> MIPHSWICEKHILWLKDYKNSSNWKLFKECWKQGQPAVVSGVHKKMNISLWKAESISLDFGDHQADLLNCKDSIISNANVKEFWDGFEEVSKRQKNKSGETVVLKLKDWPSGEDFKTMMPARYEDLLKSLPLPEYCNPEGKFNLASHLPGFFVRPDLGPRLCSAYGVVAAKDHDIGTTNLHIEVSDVVNILVYVGIAKG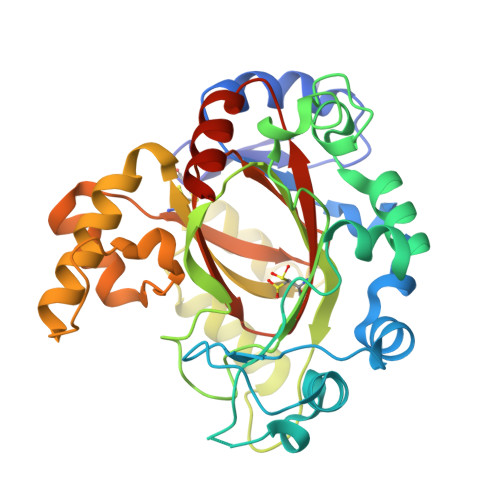NGILSKAGILKKFEEEDLDDILRKRLKDSSEIPGALWHIYAGKDVDKIREFLQKISKEQGLEVLPEHDPIRDQSWYVNKKLRQRLLEEYGVRTCTLIQFLGDAIVLPAGALHQVQNFHSCIQVTEDFVSPEHLVESFHLTQELRLLAENLYFQ> AMHQVISATTNPAKIQAILQAFEEIFGEGSCHITPVAVESGVPEQPFGSEETRAGARNRVDNARRLHPQADFWVAIEAGIDDDATFSWVVIDNGVQRGEARSATLPLPAVILDRVRQGEALGPVMSQYTGI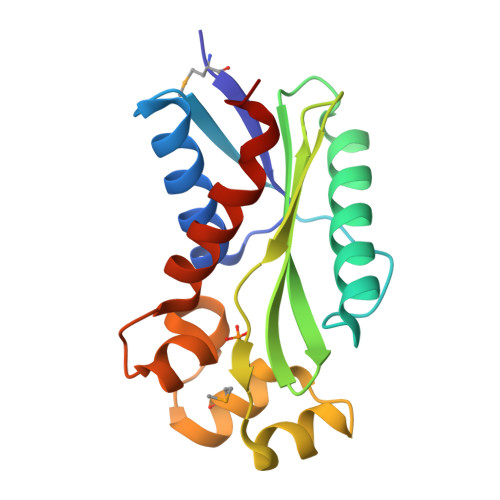DEIGRKEGAIGVFTAGKLTRSSVYYQAVILALSPFHNAVYR>GMTNLTSTHEVLAIGRLGVDIYPLQSGVGLADVQSFGKYLGGSAANVSVAAARHGHNSALLSRVGNDPFGEYLLAELERLGVDNQYVATDQTFKTPVTFCEIFPPDDFPLYFYREPKAPDLNIESADVSLDDVREADILWFTLTGFSEEPSRGTHREILTTRANRRHTIFDLDYRPMFWESPEEATKQAEWALQHSTVAVGNKEECEIAVGETEPERAGRALLERGVELAIV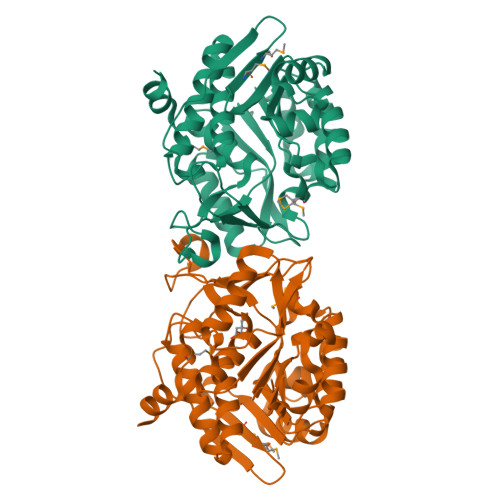KQGPKGVMAMTKDETVEVPPFFVDVINGLGAGDAFGGALCHGLLSEWPLEKVLRFANTAGALVASRLECSTAMPTTDEVEASLNQKV[4x]>[2x]MLKIATFNVNSIRSRLHIVIPWLKENKPDILCMQETKVENRKFPEADFHRIGYHVVFSGSKGRNGVAIASLEEPEDVSFGLDSEPKDEDRLIRAKIAGIDVINTYVPQGFKIDSEKYQYKLQWLERLYHYLQKTVDFRSFAVWCGDMNVAPEPIDVHSPDKLKNHVCFHEDARRAYKKILEL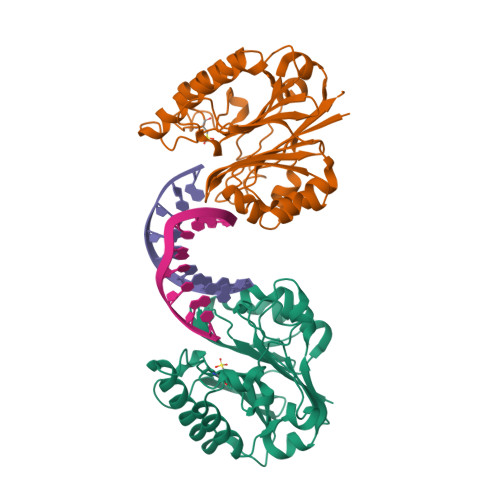GFVDVLRKIHPNERIYTFYDYRVKGAIERGLGWRGDAILATPPLAERCVDCYADIKPRLAEKPSDHLPLVAVFDV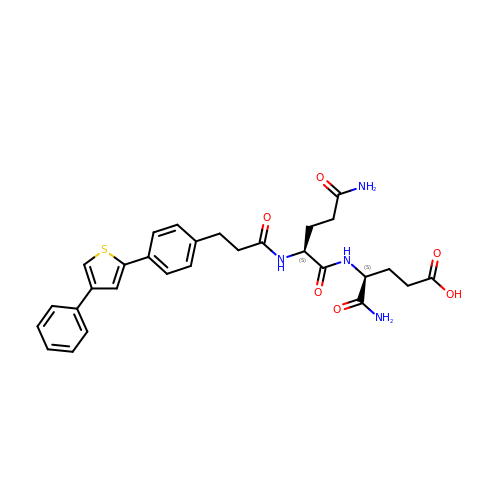N~2~-{3-[4-(4-phenylthiophen-2-yl)phenyl]propanoyl}-L-glutaminyl-L-alpha-glutamine | C29 H32 N4 O6 S | KGPPRBTYRFIDAL-GOTSBHOMSA-N>GAGGUGNNGAGCG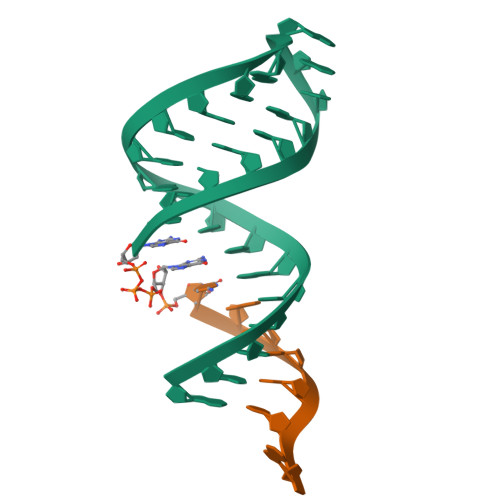CGAAAGCGCUC[3x];>[3x]XCACCUCA>[8x]MSVP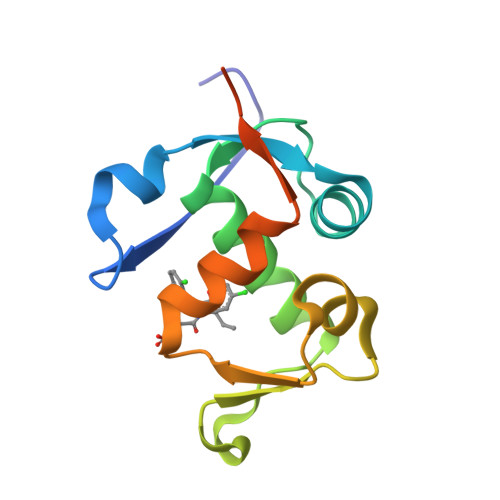TDGAVTTSQIPASEQETLVRPKPLLLKLLKSVGAQKDTYTMKEVLFYLGQYIMTKRLYDEKQQHIVYCSNDLLGDLFGVPSFSVKEHRKIYTMIYRNLVVVNQQESSDSGTSVSEN>[4x]DEGEAKEGFIEGSSLQLLTRNYYFNHDRRHASGHDSKEWAQGF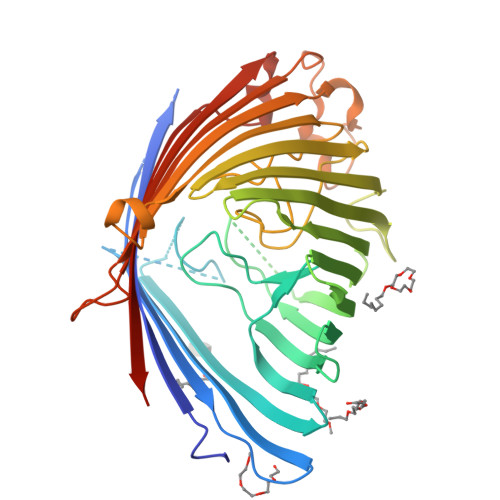IATFQSGYTPGVVGFGVDAYGMLGLKLDGGGGTGGTSILPITSPSKEGYESGKAPDEFSSGGAALKIRAFDTELKLGDQFLSNPVVAGGESRMLPQTFRGVSLTNNSFEDLTLTAGQVSFTKYYNQSGHRRLGSYYGELPGDRDSHHLSWLGGTWGGIEGFTSSLYAAELQNVWKQYYADVDYTYEIDDNWSLNPGAHYYKTVDSGDSLLGRIDNNTYSLHFAVGYRQHTVTAVLQKVNGNTPFDYINQGDSIFLDNSQQYSDFNGPNEKSWKLQYDYDFVALGVPGLSASASYSRGKLDLTRVDPDSPGYGGWYSADGKNAKHWERDLDLQYVVQGGPAKDLSLRLRWATHRGTGGYSAVDNDIDEYRVIVDYPIDVFGGHHHHHH> MHHHHHHAVRASEISRVYEAYPEKKATLYFLVLGFLALIVGSLFGPFQALNYGNVDAYPLLKRLLPFVQSYYQGLTLHGVLNAIVFTQLFAQAIMVYLPARELNMRPNMGLMWLSWWMAFIGLVVFALPLLANEATVLYTFYPPLKGHWAFYLGASVFVLSTWVSIYIVLDLWRRWKAANPGKVTPLVTYMAVVFWLMWFLASLGLVLEFVLFLLPWSFGLVEGVDPLVARTLFWWTGHPIVYFWLLPAYAIIYTILPKQAGGKLVSDPMARLAFLLFLLLSTPVGFHHQFADPGIDPTWKMIHSVLTLFVAVPSLMTAFTVAASLEFAGRLRGGRGLFGWIRALPWDNPAFVAPVLGLLGFIPGGAGGIVNASFTLDYVVHNTAWVPGHFHLQVASLVTLTAMGSLYWLLPNLTGKPISDAQRRLGLAVVWLWFLGMMIMAVGLHWAGLLNVPRRAYIAQVPDAYPHAAVPMVFNVLAGIVLLVALLLFIYGLFSVLLSRERKPELAEAPLPFAEVISGPEDRRLV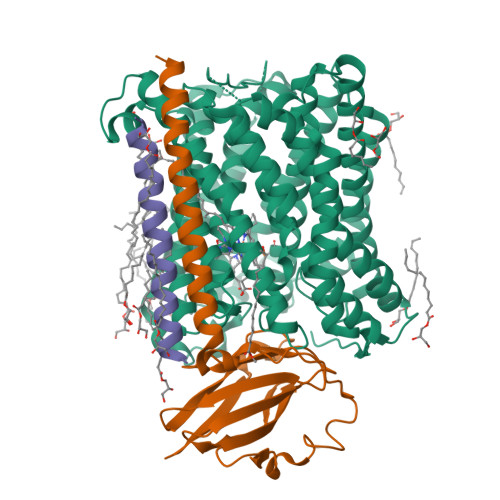LAMDRIGFWFAVAAILVVLAYGPTLVQLFGHLNPVPGWRLW;> MVDEHKAHKAILAYEKGWLAFSLAMLFVFIALIAYTLATHTAGVIPAGKLERVDPTTVRQEGPWADPAQAVVQTGPNQYTVYVLAFAFGYQPNPIEVPQGAEIVFKITSPDVIHGFHVEGTNINVEVLPGEVSTVRYTFKRPGEYRIICNQYCGLGHQNMFGTIVVKE;> MEEKPKGALAVILVLTLTILVFWLGVYAVFFARG>GTISIGCSSLIGQTLLPEVLSLYNAQFPNVEIQVQVGSTEQIKANHRDYHVMITRGNKVMNLANTHLFNDDHYFIFPKNRRDDVTKLPFIEFQADPIYINQIKQWYNDNLEQDYHATITVDQVATCKEMLISGVGVTILPEIMMKNISKEQFEFEK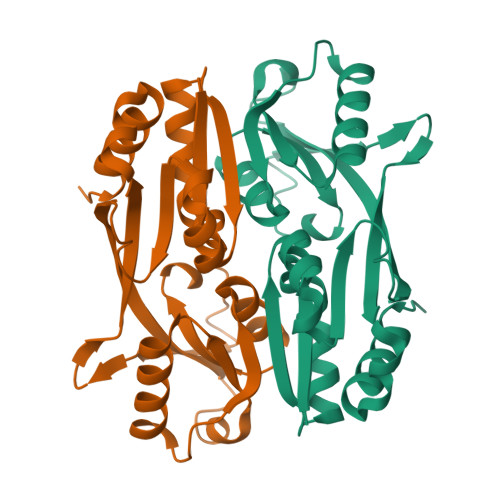VEIDNEPLIRSTFMSYDPSMLQLPQVDSFVNLMASFVEQPKA[2x]Echovirus 18 (E18), as a member of enterovirus species B, is a significant causative agent of aseptic meningitis and viral encephalitis in children. Echoviruses belong to enterovirus species B (EV-B) of the Enterovirus genus within the Picornaviridae family, which are single-stranded, positive RNA viruses (~30 nm) without a lipid envelope (nonenveloped virus). We describe the mechanism for the entry of certain EV-B serotypes by using FcRn as a two-in-one attachment-and-uncoating receptor. Protomers consist of the capsid protein (VP1, VP2, and VP3) and the smaller internal protein VP4.

Detailed characterizations of mature E18 particles, the E18/FcRn complex under physiological conditions (pH 7.4), and the E18/FcRn complex under acidic conditions (pH 5.5) were performed. To investigate whether soluble FcRn could induce E18 virion uncoating in vitro, E18 mature particles were incubated with FcRn under either neutral (pH 7.4) or acidic (pH 5.5) conditions at 37°C, and the virion morphologies were then compared by negative-stain electron microscopy. When incubating mature E18 particles with FcRn-decorated liposomes at acidic pH, the particles are first bound to the liposomes and then transformed into empty particles and released from the FcRn-decorated liposomes. When the pH of the complex was reduced to pH 5.5, rotation of the residues around the hydrophobic pocket that play a key role in stabilizing the pocket factor was observed. The rotation of these residues further displaced the pocket factor from the pocket of VP1. The release of the pocket factor was further accelerated when the pH was lowered. Accompanied by pocket factor release, FcRn dissociates from the virus particles, and the unstable virus particles initiate uncoating. The density of FcRn around the particles was observed and compared to that of the complex at pH 7.4.

> GDNQDRTVANTQPSGPSNSKEIPALTAVETGHTSQVDPSDTLQTRHVVNFHSRSESTVENFMGRAACVFMDQYKLNGEETSTDNFAVWTINVREMAQLRRKCELFTYMRFDIEMTMVITSCQDQGTQLEQDMPVLTHQIMYVPPGGPIPAKVDSYEWQTSTNPSVFWTEGNAPARMSIPFISVGNAYSLFYDGWSHFTQDGTYGYTTLNAMGKLFVRHVNKSSPHQITSTIRVYFKPKHIKAWVPRPPRLCPYINKGDVNFVVTEVTDARKSITDTPH;> SPSAEECGYSDRVRSMTLGNSTITTQESANVVVGYGEWPSYLSDKEATAEDQPTQPDVATCRFYTLESVQWEKSSPGWWWKFPEALKNMGLFGQNMHYHYLGRAGYTIHVQCNASKFHQGCLLVVCVPEAEMGCADTSTTFPATELTTEEEPHVFTSDSITGKKVQAAVCNAGMGVGVGNLTIFPHQWINLRTNNSATIVMPYINSVPMDNMFRHYNFTLMIIPFAPLNFNEGATAYVPVTVTIAPMYAEYNGLRLASTQ;> GVPVLNTPGSTQFLTSDDFQSPSAMPQFDETPEMHIPGEVRNLMEMAEVDSVVPVNNITGKTKSMEAYQIAVGTGNTDKTKPIFSFQMDPGYSSVLKRTLLGEMLNYYAHWSGSVKLTFLFCGSAMATGKLLISYSPPGASVPSSRKDAMLGTHIIWDIGLQSSCVLCVPWISQSHYRMVQQDPYTSAGYITCWYQTNIVVPPGAPTSCDVLCFASACNDFSVRLLRDTPFMAQPGKLQ;> MGAQVSTQKTGAHETSLNAKGNSIIHYTNINFYKDAASSASNRQELQQDPGKFTDPVKDLMVKTLPALN>MARKYFVAANWKCNGTLESIKSLTNSFNNLDFDPSKLDVVVFPVSVHYDHTRKLLQSKFSTGIQNVSKFGNGSYTGEVSAEIAKDLNIEYVIIGHFERRKYFHETDEDVREKLQASLKNNLKAVVCFGESLEQREQNKTIEVITKQVKAFVDLIDNFDNVILVYEPLFAIGTGKTATPEQAQLVHKEIRKIVKDTCGEKQANQIRILYGGSVNTENCSSLIQQEDIDG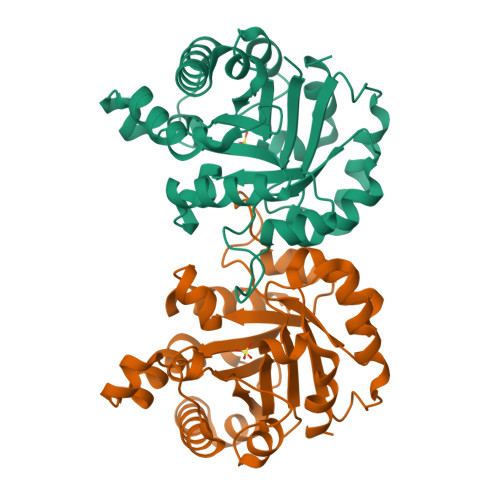FLVGNASLKESFVDIIKSAM[4x]>[2x]MTEDRLSAEDKKFLEVERALKEAALNPLRHATEELFGDFLKMENITEICYNGNKVVWVLKNNGEWQPFDVRDRKAFSLSRLMHFARCCASFKKKTIDNYENPILSSNLANGERVQIVLSPVTVNDETISISIRIPSKTTYPHSFFEEQGFYNLLDNKEQAISAIKDGIAIGKNVIVCGGTGSGKTTYIKSIMEFIPKEERIISIEDTEEIVFKHHKNYTQLFFGGNITSADCLKSCLRMRPD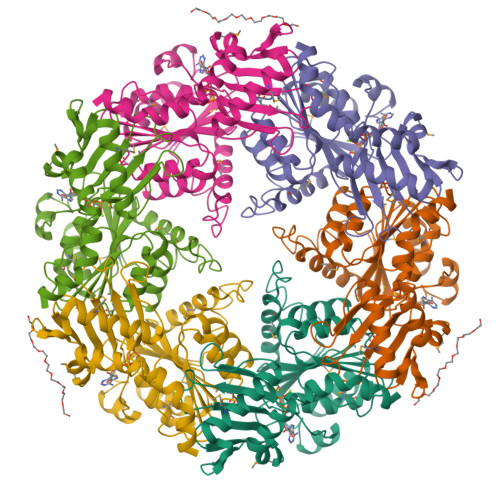RIILGELRSSEAYDFYNVLCSGHKGTLTTLHAGSSEEAFIRLANMSSSNSAARNIKFESLIEGFKDLIDMIVHINHHKQCDEFYIKHR1-(5-{2-[(1-methyl-1H-pyrazolo[4,3-d]pyrimidin-7-yl)amino]ethyl}-1,3-thiazol-2-yl)-3-[3-(trifluoromethyl)phenyl]urea 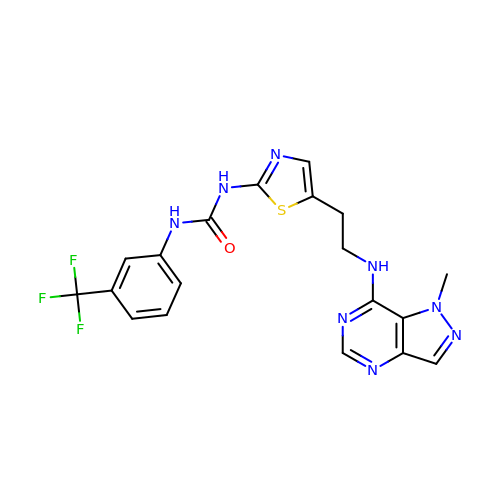| C19 H17 F3 N8 O S | UOLCZAFAGDOUFX-UHFFFAOYSA-N> MDPIGINKVLDHLAPSELIKPVKSCHNKPSVLVLDDRIVDAATKDLYVNGFQEEIQYQNPTPENLQHMFHQGIEILDSARMINVTHLALWKPSSFKLGNPVDFALDDNYDTFWQSDGGQPHQLDIMFSKRMDICVMAIFFSMIADESYAPSLV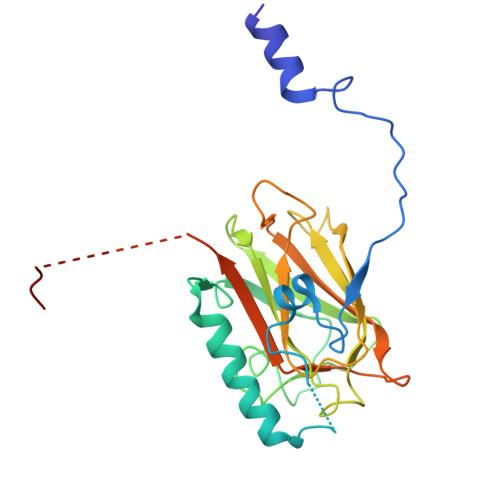KVYAGHSPSDARFYKMLEVRNVNGWVALRFLDNREDDQLLKCQFIRLLFPVNHENGKDTHLRGIRLYVPSNEPHQDTHEWAQTLPETNNVFQDAILR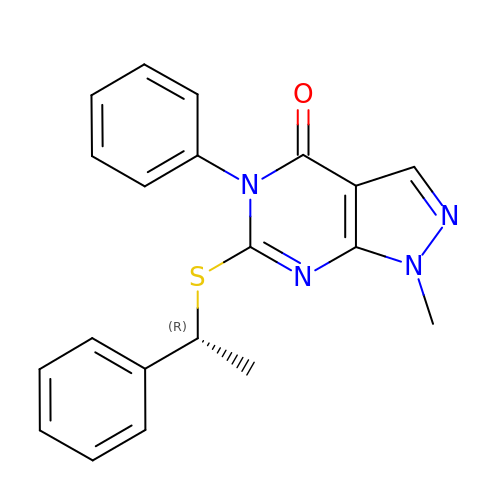1-methyl-5-phenyl-6-{[(1R)-1-phenylethyl]sulfanyl}-1,5-dihydro-4H-pyrazolo[3,4-d]pyrimidin-4-one | C20 H18 N4 O S | JNPNRKXZLIGUCT-CQSZACIVSA-N>[2x]DRVYIHPFHLLYYSKSTCAQLENPSVETLPEPTFEPVPIQAKTSPVDEKTLRDKLVLATEKLEAEDRQRAAQVAMIANFMGFRMYKMLSEARGVASGAVLSPPALFGTLVSFYLG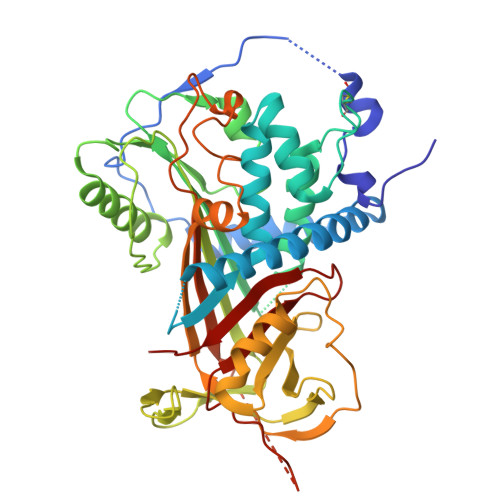SLDPTASQLQVLLGVPVKEGDCTSRLDGHKVLTALQAVQGLLVTQGGSSSQTPLLQSTVVGLFTAPGLRLKQPFVESLGPFTPAIFPRSLDLSTDPVLAAQKINRFVQAVTGWKMNLPLEGVSTDSTLFFNTYVHFQGKMRGFSQLTGLHEFWVDNSTSVSVPMLSGTGNFQHWSDAQNNFSVTRVPLGESVTLLLIQPQCASDLDRVEVLVFQHDFLTWIKNPPPRAIRLTLPQLEIRGSYNLQDLLAQAKLSTLLGAEANLGKMGDTNPRVGEVLNSILLELQAGEEEQPTESAQQPGSPEVLDVTLSSPFLFAIYERDSGALHFLGRVDNPQNVV> MASMTGGQQMGRDQAGITGTWYNQLGSTFIVTAGADGALTGTYESAVGNAESRYVLTGRYDSAPATDGSGTALGWTVAWKNNYRNAHSATT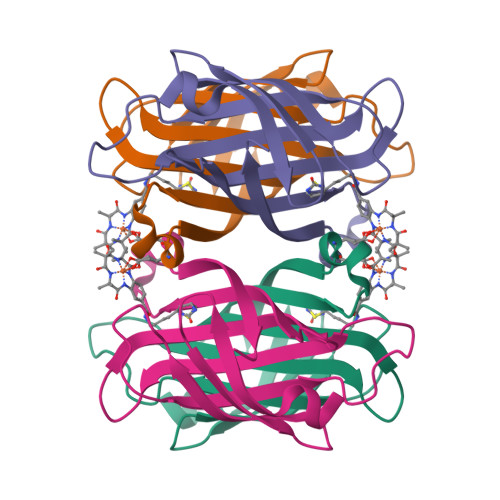WSGQYVGGAEARINTQWLLTRGTTEANAWESTLVGHDTFTKVKPSAASIDAAKKAGVNNGNPLDAVQQ CYSTEINE | C3 H7 N O2 S | 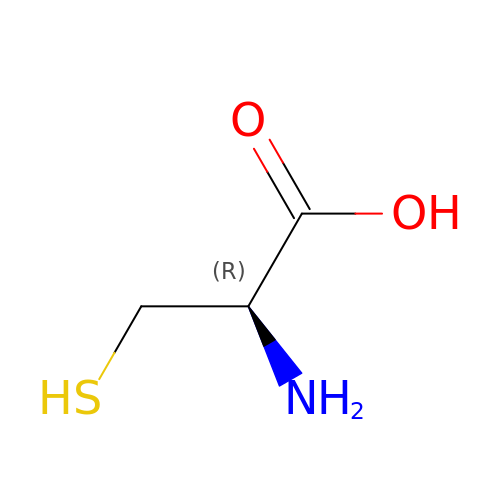XUJNEKJLAYXESH-REOHCLBHSA-N8-azido-1-((1S,2S,3S,4S,5R,6S)-2,3,4-trihydroxy-5-(hydroxymethyl)-7-azabicyclo[4.1.0]heptan-7-yl)octan-1-one 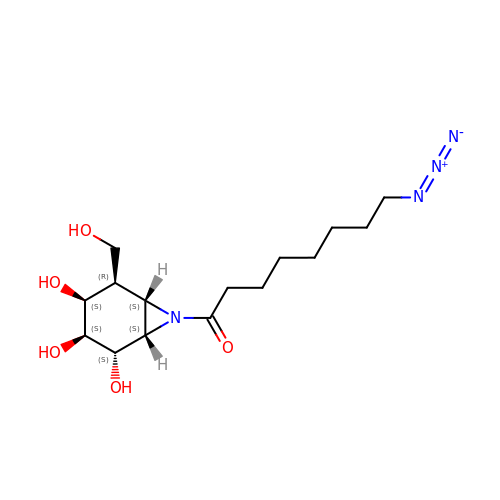| C15 H26 N4 O5 | BVEYUFNXLOTLDG-DWDHYAMMSA-N> MEILYTGASESLHSTILKALLERIDLGDTFISDNYTRWQATERYYMMYKIPNKKDKAAIEKWNKGDTDFKSLVMPYSYAQLMTAHAYMVNVFLNRDPIFQTDSLNGDGTERELALESMLQYQVKAGEMEPSLLVWFMDALRYGVGVLGDYWEEHVFHQTVFEEEEEIIDGVPTGNMKKVKKTRVVKGYEGCKTFNVMVYDFIPDPRVALCKYQEGEFFGRRLDLNVLDLKKGAKFGKYFNVEHAEALVAASKEEMYRRDPSIGQQRSLKDSTMTPKGKQVGDISCVEIFVRLVPKDWGLGDSEFPEMWVFTVADKKYIVAAEPVNTLDDKFPFHILECEIDGYMNKSRGLLEISAPM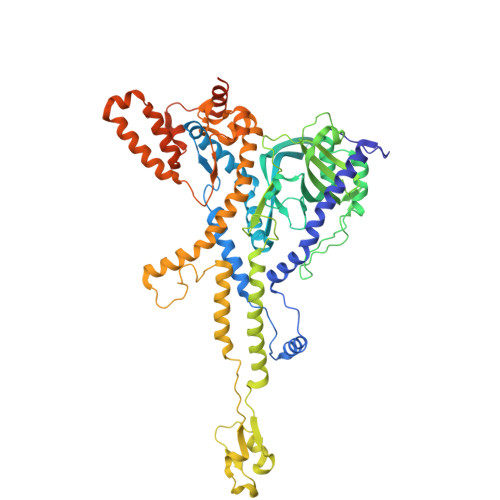NDILTWLFDSHMYNKRQIMNNQFIGDPSALVVKDVESKEPGKFIRLRPTAYGRDVRSIISQLPVTDVTAQNIQDVQVVERNMQRIVGVNDDVAGQSSPSSRRSATEFRGTTSFASSRLANLAYFFSVTGFRSLAKSLIVKTQQLYTVEMKVKVAGDNIKGAQSIIVKPEDISGQFDIMPVDGTLPVDRMAQAQFWMQIMSMVAGNPVLGAEYRLGDIFSYTARLAGLKGIDKMKIRILDDDQILALILAQQKGGADVQPTGQPTTQGVGNPTGVNEPAPSVTQGTPGLSGLQALM> REFPPPNPDPKFESKAALLAARGPEELLCFTERLEDLVCFWEEAASAGVGPGQYSFSYQLEDEPWKLCRLHQAPTARGAVRFWCSLPTADTSSFVPLELRVTAASGAPRYHRVIHINE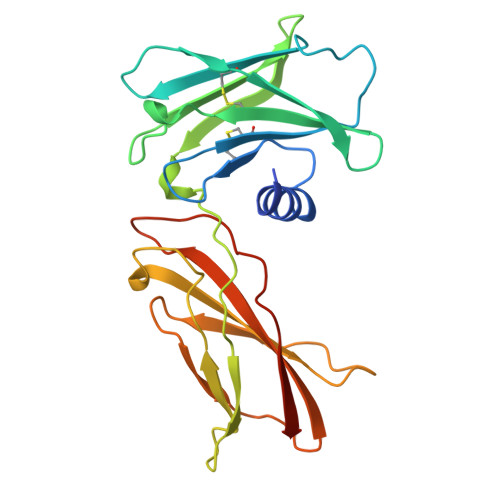VVLLDAPVGLVARLADESGHVVLRWLPPPETPMTSHIRYEVDVSAGQGAGSVQRVEILEGRTECVLSNLRGRTRYTFAVRARMAEPSFGGFWSEWSEPVSLLTPSDLDP>[4x]MAETDGSIPLIPVRMLNEHVYCPRLAYLMWVQGEFSHNEFTVDGVIRHRRVDAGGGVLPSETQEDSRIHARSVSLSSERLGITAKIDLVEGEGAYVSPVDYKRGKRPHVAGGAYEPERVQLCAQGLLLREHGFASDGGALYFVASRERVPVAFDDELIGRTLAAIDEMGRTALSGTMPPPLEDSPKCPRCSLVGICLPDEVRFLSHLSVEPRPIIPADGRGLPLYVQSPKAYVRKDGDCLVIEEERVRVAEARLGETSQVALFGNATLTTAALHECLRREIPVTWLSYGGWFMGHTVSTGHRNVETRTYQYQRSFDPETCLNLARRWIVAKIANCRTLLRRNWRGEGDEAKAPPGLLMSLQDDMRHAMRAPSLEVLLGIEGASAGRYFQHFSRMLR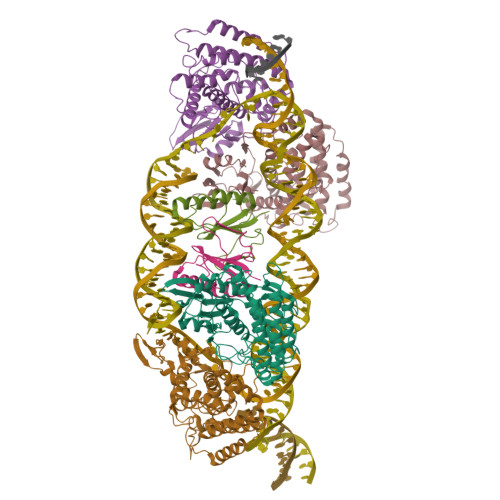GGDGEGMGFDFTTRNRRPPKDPVNALLSFAYAMLTREWTVALAAVGLDPYRGFYHQPRFGRPALALDMMEPFRPLIADSTVLMAINNGEIRTGDFVRSAGGCNLTDSARKRFIAGFERRMEQEVTHPIFKYTISYRRLLEVQARLLTRYLSGEIPAYPNFVTR;>MEHLYIVSYDIRNQRRWRRLFKTMHGFGCWLQLSVFQCRLDRIRIIKMEAAINEIVNHAEDHVLILDLGPAENVKPKVSSIGKTFDPILRQAVIV[2x]> SMSLNIITVTLNMEKYNFLGISIVGQSNERGDGGIYIGSIMKGGAVAADGRIEPGDMLLQVNDMNFENMSNDDAVRVLRDIVHKPGPIVLTVAKCW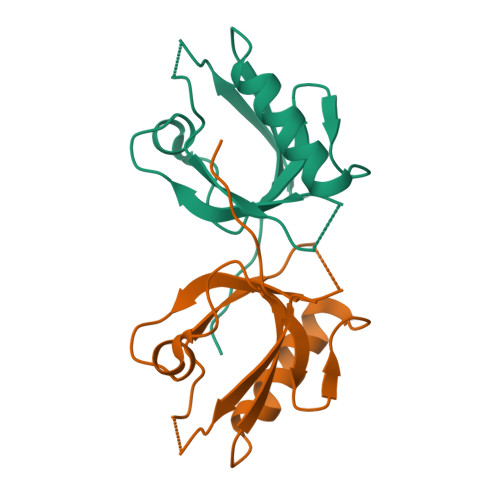ETSV> CTVGPDYRTPDTAAAKIDATASKPYDRSRFE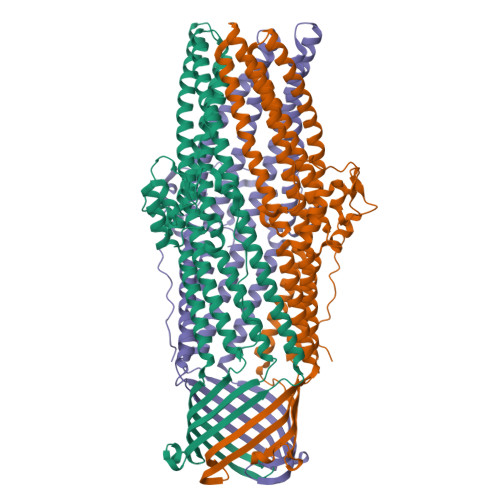SLWWKQFDDPTLNQLVEQSLSGNRDLRVAFARLRAARALRDDVANDRFPVVTSRASADIGKGQQPGVTEDRVNSERYDLGLDSAWELDLFGRIRRQLESSDALSEAAEADLQQLQVSLIAELVDAYGQLRGAQLREKIALSNLENQKESRQLTEQLRDAGVGAELDVLRADARLAATAASVPQLQAEAERARHRIATLLGQRPEELTVDLSPRDLPAITKALPIGDPGELLRRRPDIRAAERRLAASTADVGVATADLFPRVSLSGFLGFTAGRGSQIGSSAARAWSVGPSISWAAFDLGSVRARLRGAKADADAALASYEQQVLLALEESANAFSDYGKRQERLVSLVRQSEASRAAAQQAAIRYREGTTDFLVLLDAEREQLSAEDAQAQAEVELYRGIVAIYRSLGGGWQPSAGSHHHHHH The LftR protein transcriptionally regulates the expression of the lmo0980 gene, which encodes a putative multidrug resistance transporter, LieAB (Listerial importer of ethidium bromide as artificial substrate), and facilitates the export of toxic chemicals from the cytoplasm to the extracellular space. LftR contains 108 residues and is expected to belong to the PadR-2 subfamily. As transcriptional regulators, PadR family members commonly contain a winged helix-turn-helix (wHTH) motif to interact with operator DNA. The apparent molecular weights of both LftR proteins were estimated to be 20–24 kDa, whereas the calculated molecular weights are ~12 kDa, indicating that LftR forms a homodimer in solution regardless of construct designs.

The LftRCtH protein was purified with the C-terminal His6 tag. As a first step in the understanding of LftR at a molecular level, LftRΔNtH and LftRCtH structures were determined and refined at 2.3 and 2.8 Å resolutions, respectively. The monomeric structures of LftRΔNtH and LftRCtH are mostly similar, but local structural differences are observed at the H0 helix and the β1 and β2 strands. Residues 4–8 form an α-helix (H0 helix) in the LftRΔNtH, whereas the corresponding region of LftRCtH adopts an extended coil structure, indicating the flexible nature of the LftR N-terminal residues. Thus, the LftRCtH structure exhibits a longer loop (residues 66–72) between the β1 and β2 strands than the LftRΔNtH structure (residues 67–69). When the dimeric structures of LftRΔNtH and LftRCtH were superposed using the wHTH motifs of subunit A, the structures of subunit A were overlaid well, but those of subunit B were not superimposable due to severe positional displacements in the quaternary structures. The dimer-forming H1ʹ helix and its neighboring wHTHʹ motif of the LftRΔNtH structure positionally differ from those of the LftRCtH structures with rotation up to ~23° and translation up to ~9 Å. As a result, the inter-wHTH distance of the LftRCtH dimer (~81 Å) is ~11 Å longer than that of the LftRΔNtH dimer (~70 Å). The cavity of the LftRCtH dimer structure (cavity surface, ~277 Å2; internal volume, ~148 Å3) is larger than the cavity of the LftRΔNtH dimer (cavity surface, ~157 Å2; internal volume, ~83 Å3) probably due to conformational changes in the dimerization residues. Noticeably, the comparative analysis of the LftRΔNtH and LftRCtH structures indicated that the cavity of LftR is flexible and can be modulated by intersubunit reorganization.

>ALKGSLEGMILERISRGETYGYEITKYLNDLGFDEIVEGTVYTILVRLEKKGLVEIEKKKSELGPPRKFYTLSPAGEEELAIFWKRWDFIQGKIMQVK[2x]> MKEFGDSLSLEILQIIKESQQQHGLRHGDFQRYRGYCSRRQRRLRKTLNFKMGNRHKFTGKKVTEELLTDNRYLLLVLMDAERAWSYAMQLKQEANTEPRKRFHLLSRLRKAVKHAEELERLCESNRVDAKTKLEAQAYTAYLSGMLRFEHQEWKAAIEAFNKCKTIYEKLASAFTEEQAVLYNQRVEEISPNIRYCAYNIGDQSAINELMQMRLRSGGTEGLLAEKLEALITQTRAKQAATMSEVEWRGRTVPVKIDKVRIFLLGLADNEAAIVQAESEETKERLFESMLSECRDAIQVVREELKPDQKQRDYILEGEPGKVSNLQYLHSYLTYIKLSTAIKRNENMAKGLQRALLQQQPEDDSKRSPRPQDLIRLYDIILQNLVELLQLPGLEEDKAFQKEIGLKTLVFKAYRCFFIAQSYVLVKKWSEALVLYDRVLKYANEVNSDAGAFKNSLKDLPDVQELITQVRSEKCSLQAAAILDANDAHQTETSSSQVKDNKPLVERFETFCLDPSLVTKQANLVHFPPGFQPIPCKPLFFDLALNHVAFPPLEDKLEQKTKSGLTGYIKGIFGFRS;> SNAMASGGSGGVSVPALWSEVNRYGQNGDFTRALKTVNKILQINKDDVTALHCKVVCLIQNGSFKEALNVINTHTKVLANNSLSFEKAYCEYRLNRIENALKTIESANQQTDKLKELYGQVLYRLERYDECLAVYRDLVRNSQDDYDEERKTNLSAVVAAQSNWEKVVPENLGLQEGTHELCYNTACALIGQGQLNQAMK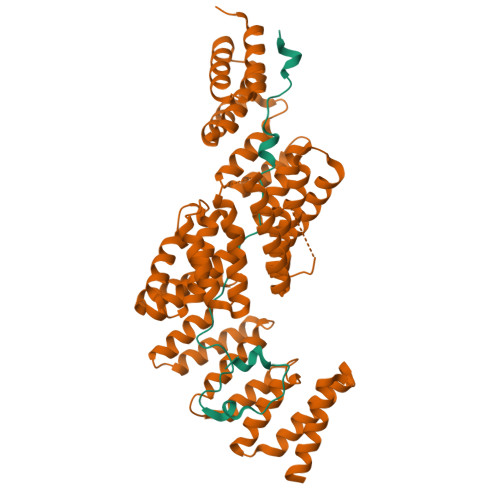ILQKAEDLCRRSLSEDTDGTEEDPQAELAIIHGQMAYILQLQGRTEEALQLYNQIIKLKPTDVGLLAVIANNIITINKDQNVFDSKKKVKLTNAEGVEFKLSKKQLQAIEFNKALLAMYTNQAEQCRKISASLQSQSPEHLLPVLIQAAQLCREKQHTKAIELLQEFSDQHPENAAEIKLTMAQLKISQGNISKACLILRSIEELKHKPGMVSALVTMYSHEEDIDSAIEVFTQAIQWYQNHQPKSPAHLSLIREAANFKLKYGRKKEAISDLQQLWKQNPKDIHTLAQLISAYSLVDPEKAKALSKHLPSSDSMSLKVDVEALENSAGATYIRKKGGKVTGDSQPKEQGQGDLKKKKKKKKGKLPKNYDPKVTPDPERWLPMRERSYYRGRKKGKKKDQIGKGTQGATAGASSELDASKTVSSPPTSPRPGSAATVSASTSNIIPPRHQKPAGAPATKKKQQQKKKKGGKGGW>MRGSHHHHHHGSMDRPFIFINSAMSADGKLSTKERKQVKISGKLDFERMDELRAHADAIMVGIGTVLADDPSLTVKSPERKAARKAAGKSENPVRVVVDSSARTPLNADIFKKGEGLRIIAVSNSAPEEKIRMLEEKALVIKTGAFRVDLTELAAKLKEMGINSLMVEGGATLNWGMLSAGLVDEVYTFVGNLIIGG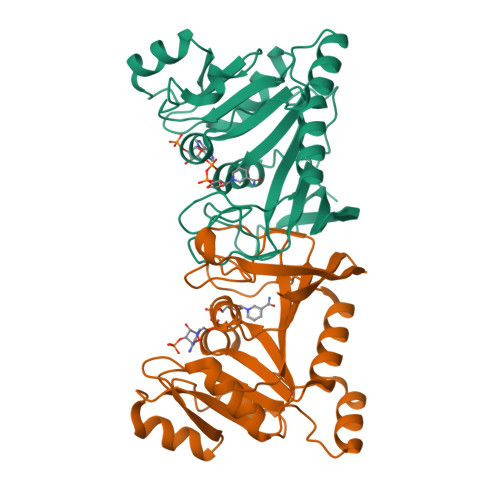KTAPTFTDGEGFTENELLGLELSSAEKIEDGILLKWKVKGKKN[6x]> NARRKLKG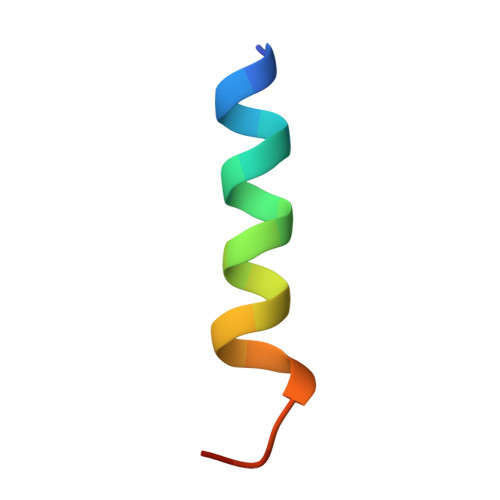AILTTMLATRNFSG> MKLIDKLPSFDRNYIVEEIQGAYDTELNILKEDIDDTFNQLFVDTATWGLDMWEDILCIEKKELDFDTRRSNIKAKMRSRGTSTIEVIKSICEAYTKSETDIKVYSDEFTFVLSFIANNCDYKTLLDCSDMIERVKPAHLLHYLEPIILDKSMVYCGGGMVCSEEVKVHPYFEPIIKCSAVVNCGAGMISREEIKVYPLSIKCIENNCKINIAIA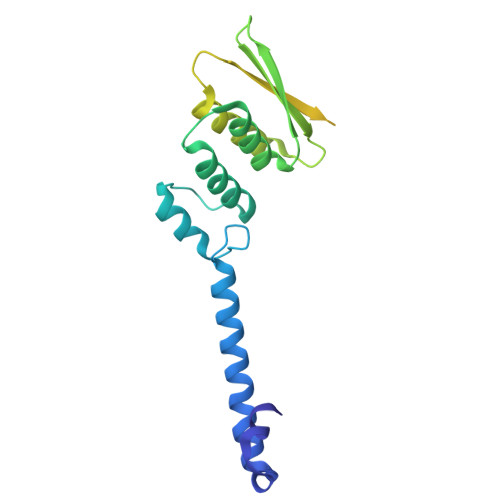NDTGVENVVVYPKSEVV> GAGVSRQNVGTH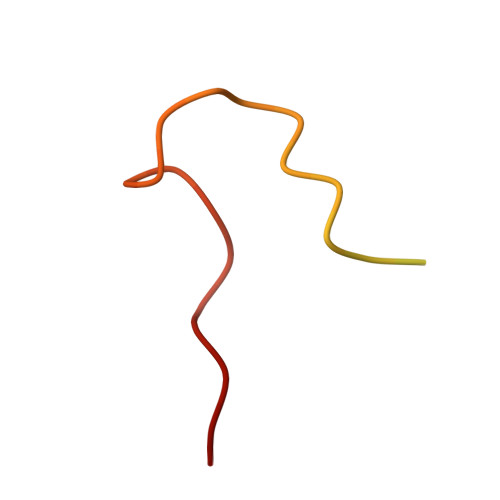STQNSVSNGSSLNYFNINYFKDAASSGASRLD>MAELLLGVNIDHIATLRNARGTAYPDPVQAAFIAEQAGADGITVHLREDRRHITDRDVRILRQTLDTRMNLEMAVTEEMLAIAVETKPHFCCLVPEKRQEVTTEGGLDVAGQRDKMRDACKRLADAGIQVSLFIDADEEQIKAAAEVGAPFIEIHTGCYADAKTDAEQAQELARIAKAA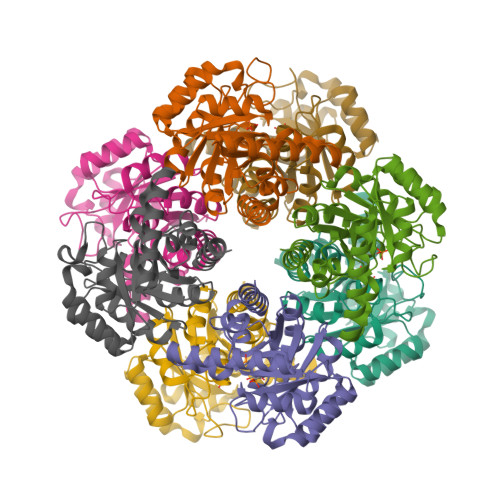TFAASLGLKVNAGHGLTYHNVKAIAAIPEMHELNIGHAIIGRAVMTGLKDAVAEMKRLMLEARG[8x]A potential new target for Chagas' disease chemotherapy is sterol 14α-demethylase (CYP51), a cytochrome P450 heme thiolate-containing enzyme which is involved in biosynthesis of membrane sterols in all biological kingdoms from bacteria to animals. Azoles block CYP51 activity, resulting in decline of the normal complement of endogenous sterols and accumulation of various 14α-methyl sterols with cytostatic or cytoxic consequences. Based upon crystal structures of CYP51 of M. tuberculosis (CYP51Mt), three of the thirteen active site residues, Y76, F83, and H259 (numbering according to CYP51Mt), are invariant throughout the cyp51 gene family. To verify this assumption, we determined the binding modes of second generation compounds containing the N-[4-pyridyl]-formamide moiety by determining their co-crystal structures with CYP51Mt.

Compound 7 was not found in the CYP51Mt active site in the crystal, which is consistent with lack of spectrally detectable binding. Compounds 8 (3-{[(4-methylphenyl)sulfonyl]amino}propylpyridin-4-ylcarbamate), 9 (cis-4-methyl-N-[(1S)-3-(methylsulfanyl)-1-(pyridin-4-ylcarbamoyl)propyl]cyclohexanecarboxamide), and 11 (N-[(1S)-2-methyl-1-(pyridin-4-ylcarbamoyl)propyl]cyclohexanecarboxamide), were observed bound in the CYP51Mt active site as predicted, through the coordination of the heme iron via a lone pair of aromatic nitrogen electrons of the N-[4-pyridyl]-formamide moiety (highlighted in gray in Fig. 2) and interactions with the invariant residues Y76 and H259. Functional groups other than the N-[4-pyridyl]-formamide moiety in compounds 9 and 11 either were accommodated in the species-specific cavity or else protruded through the opening of the active site toward bulk solvent. H259 hydrogen-bonded to the carbonyl oxygen in both compounds, while interactions with Y76 were mediated by two similarly positioned water molecules. The residual Fo-Fc electron density map suggested two alternative conformations for compounds 11 and 9, designated by pink and cyan respectively in Figures 4A and 4B. In the CYP51Mt-compound 11 complex, the cyclohexane ring protruded toward the bulk solvent, barely interacting with the protein in two alternative conformations. Together with the limited interactions of the isopropyl moiety, this lack of contact explains the low binding affinity of 11. In both complexes, a portion of the BC-region was disordered and missing from the electron density map. Although racemic mixtures were used for co-crystallization, only one enantiomer of each compound was found in the active site. No binding was observed for compound 7, while the KD for compound 11 exceeded 100 µM, indicating weak binding.

> MSAVALPRVSGGHDEHGHLEEFRTDPIGLMQRVRDELGDVGTFQLAGKQVVLLSGSHANEFFFRAGDDDLDQAKAYPFMTPIFGEAVVFDASPERRKEMLHNAALRGEQMKGHAATIEDQVRRMIADWGEAGEIDLLDFFAELTIYTSSACLIGKKFRDQLDGRFAKLYHELERGTDPLAYVDPYLPIESFRRRDEARNGLVALVADIMNGRIANPPTDKSDRDMLDVLIAVKAETGTPRFSADEITGMFISMMFAGHHTSSGTASWTLIELMRHRDAYAAVIDELDELYGDGRSVSFHALRQIPQLENVLKETLRLHPPLIILMRVAKGEFEVQGHRIHEGDLVAASPAISNRIPEDFPDPHDFVPARYEQPRQEDLLNRWTWIPFGAGRHRCVGAAFAIMQIKAIFSVLLREYEFEMAQPPESYRNDHSKMVVQLAQPAAVRYRRRTGVHHHH> MGHHHHHHHHHHSSGHIEGRHMFSKNAVKLHATPPSVAAPPTGAPEVAAERLEPRVEEKDGYWILKEQFRKGINPQEKVKIEKEPMKLFMENGIEELAKIPIEEIDQSKLTKDDIDVRLKWLGLFHRRKNQYGRFMMRLKLPNGVTTSAQTRYLASVIRKYGKEGCADITTRQNWQIRGVVLPDVPE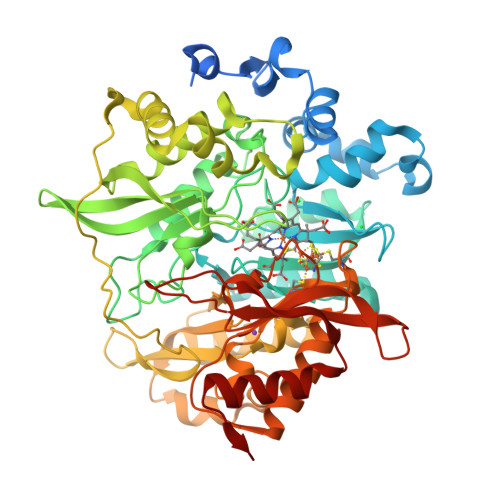ILKGLAEVGLTSLQSGMDNVRNPVGNPLAGIDPEEIVDTRPYTNLLSQFITGNSRGNPAVSNLPRKWNPCVVGSHDLYEHPHINDLAYMPATKDGRFGFNLLVGGFFSAKRCDEAIPLDAWVPADDVVPVCRAILEAFRDLGFRGNRQKCRMMWLIDELGVEGFRAEVEKRMPQQQLERASPEDLVQKQWERRDYLGVHPQKQEGYSFIGLHIPVGRVQADDMDELARLADEYGSGEIRLTVEQNIIIPNIETSKIEALLKEPVLSTFSPDPPILMKGLVACTGNQFCGKAIIETKARSLKITEEVQRQVSLTKPVRMHWTGCPNTCAQVQVADIGFMGCLTRDKNGKTVEGADVFLGGRIGSDSHLGEVYKKAVPCDDLVPLVVDLLVNNFGAVPR As a ubiquitous herpesvirus with a seroprevalence of more than 50% in adults, human cytomegalovirus (HCMV) encodes four viral GPCRs (vGPCRs) including US27, US28, UL33 and UL78. The first three show about 30% homology to chemokine receptors (e.g., CXCR3, CX3CR1, CCR10 and CXCR1), whereas UL78 displays negligible homology to any endogenous receptors. While previous studies suggest that US27, UL33 and UL78 regulate viral replication or reactivation, there is no existing evidence demonstrating their interactions with chemokines; thus, they are classified as orphan receptors. In this study, we report the cryo-EM structure of UL78 and unveil a novel form of GPCR oligomerization unseen before — a homotrimeric architecture, thereby broadening our knowledge about GPCR structures.

When the receptor was expressed solely, only the trimeric form rather than monomer was detected in non-denaturing gel. After sample preparation, cryo-EM data collection and single-particle analysis, a 3D consensus density map was reconstructed with a global resolution of 3.12 Å, enabling model building for all seven transmembrane helices (TMs), three intracellular loops (ICLs) and extracellular loops (ECLs) 1 and 2. The overall structure of UL78 comprises a homotrimer along the 3-fold symmetry axis with each protomer closely interacting with the other two. Three protomer structures share a highly conserved conformation with Cα root mean square deviation (RMSD) values of 0.50–0.56 Å and adopt a unique conformation that distinct from both active and inactive CXCR3 structures (Cα RMSD values of 1.06 Å and 1.28 Å, respectively). Specifically, the inward movements (10.0 Å and 13.1 Å) of ICL2 and the intracellular end of TM7 fulfill the receptor intracellular crevice, thereby hindering the insertion of the C-terminus of Gαi. This intracellular closure is achieved by various interactions, including D133TM3−R134TM3−E148ICL2 salt bridges, D143ICL2−R301H8 salt bridge, R69ICL1−W145ICL2−H146ICL2−H147ICL2−R142ICL2 stackings, F127TM3−F239TM6−Y240TM6−F294TM7−F298TM7 stackings and I138TM3−V229TM6 hydrophobic contacts. Looking at the extracellular side, the top of orthosteric ligand-binding pocket was significantly covered by the inward-folded ECL2, while the latter forms many polar contacts with the surrounding TMs. Although the ECL2 of BILF1 and US27 also forms a lid that caps the chemokine-binding pocket, the extracellular architecture of UL78 is more compact, and lacks the participation of ECL3 or interaction with the N-terminus. UL78 forms a stable homotrimeric architecture through an extensive interface covering TMs 3–6, ICL1 and ICL2 with a large interface area (7956 Å2). A central triangle in the trimer was formed by the tightly packed TM5 from three protomers, while the extracellular and intracellular halves of TM5 were further clasped by TM4 and TM3 from one neighboring protomer, respectively.

>SADRAASDLLIGMFGSVSLVNLLTIIGCLWVLRVTRPPVSVMIFTWNLVLSQFFSILATMLSKGIMLRGALNLSLCRLVLFVDDVGLYSTALFFLFLILDRLSAISYGRDLWHHETRENAGVALYAVAFAWVLSIVAAVPTAATGSLDYRWLGCQIPIQYAAVDLTIKMWFLLGAPMIAVLANVVELAYSDRRDHVWSYVGRVCTFYVTCLMLFVPYYCFRVLRGVLQPASAAGTGFGIMDYVELATRTLLTMRLGILPLFIIAFFSREPTKDLDDSFDYLVERC[3x]> MHHHHHH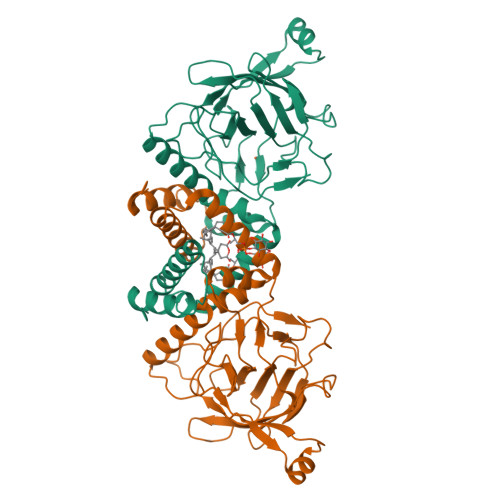NRQQIDALVKQMNVDTAKGPVDERIQQVVVRLLGDLFQAIEDLDIQPSEVWKGLEYLTDAGQANELGLLAGGLGLEHYLDLRADEADAKAGITGGTPRTIEGPLYVAGAPESVGFARMDDGSESDKVDTLIIEGTVTDTEGNIIEGAKVEVWHANSLGNYSFFDKSQSDFNLRRTILTDVNGKYVALTTMPVGYGCPPEGTTQALLNKLGRHGNRPSHVHYFVSAPGYRKLTTQFNIEGDEYLWDDFAFATRDGLVATATDVTDEAEIARRELDKPFKHITFNVELVKEAEAAPSSEVERRRASA> GSIYTFNELVVLDYPHKDRALRYLERLRDDTGIKKIMDSHRWTVPLLSEMDPAEHTRHDSKTLGLNHNQGAHIELRLRTDRYDGFRDYKTVKSTLIHELTHNVHGEHDSSFWELFRQLTKEADAADL

Covalent DNA-protein crosslinks (DPCs) are toxic DNA lesions that interfere with essential chromatin transactions, such as replication and transcription. In yeast, DPC proteolysis is catalyzed by the metalloprotease Wss1, which permits replication in the presence of DPCs and provides resistance toward DPC-inducing agents. Intriguingly, Wss1 is a DNA-dependent protease that degrades DNA-bound substrates in vitro irrespective of identity. Spartan (SPRTN, DVC1) is distantly related to yeast Wss1, displays a similar domain organization, and shares a common evolutionary origin (Stingele et al., 2015).

To gain insights into how this feat is achieved, we sought to obtain structural information on this protease family. We focused on the protease domain, as the presumably highly dynamic C-terminal tail containing various protein-protein interaction motifs interferes with crystallization of full-length protein. While most proteins were insoluble, we were able to purify the protease domain of Wss1b, one of the two SPRTN homologs in Schizosaccharomyces pombe. An X-ray fluorescence spectrum of crystals obtained at the synchrotron revealed the presence of nickel as the only heavy-metal atom. An anomalous dataset at the Ni2+ edge (z = 1.4854) confirmed that this ion occupies the active site of the enzyme, where it replaced the catalytic zinc presumably during the Ni2+-affinity chromatography. The overall architecture depicted a compact protease domain consisting of four tightly packed α helices and a four-stranded antiparallel β sheet. The catalytic center was formed by three histidines, as well as two water molecules and one oxygen molecule, that jointly coordinated the active site metal ion by forming a distorted octahedron. Intriguingly, the catalytic center comprising the metal-binding motif was highly solvent exposed. This together with the absence of an obvious substrate-binding cleft or region could explain the promiscuity of SPRTN/Wss1 proteases with respect to substrate identity. Our structural data further highlighted the need to restrain the protease activity of the SPRTN/Wss1 family since the catalytic center is solvent exposed and bears few signs of specificity-generating features.>[2x]MAKLLIMSIVSFCFIFLLLLFFRYILKRYFNYMLNYKVWYLTLLAGLIPFIPIKFSLFKFNNVNNQAPTVESKSHDLNHNINTTKPIQEFATDIHKFNWDSIDNICTVIWIVLVIILSFKFLKALLYLKYLKKQSLYLNENEKNKIDTILFNHQYKKNIVI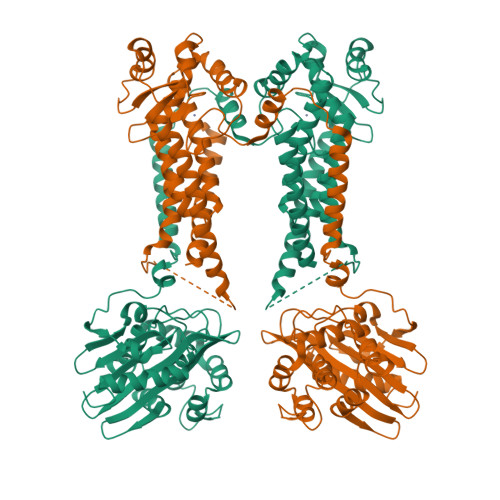RKAETIQSPITFWYGKYIILIPSSYFKSVIDKRLKYIILHEYAHAKNRDTLHLIIFNIFSIIMSYNPLVHIVKRKIIHDNEVEADRFVLNNINKNEFKTYAESIMDSVLNVPFFNKNILSHSANGKKSLLKRRLINIKEANLKKQSKLILIFICIFTFLLMVIQSQFLMGQSITDYNYKKPLHNDYQILDKSKIFGSNSGSFVMYSMKKDKYYIYNEKESRKRYSPNSTYKIYLAMFGLDRHIINDENSRMSWNHKHYPFDAWNKEQDLNTAMQNSVNWYFERISDQIPKNYTATQLKQLNYGNKNLGSYKSYWMEDSLKISNLEQVIVFKNMMEQNNHFSKKAKNQLSSSLLIKKNEKYELYGKTGTGIVNGKYNNGWFVGYVITNHDKYYFATHLSDGKPSGKNAELISEKILKEMGVLNGQELALVPRGSSAHHHHHH>[4x]MGGSEIPMSEKTTKGVQLLRGDPKKAIVR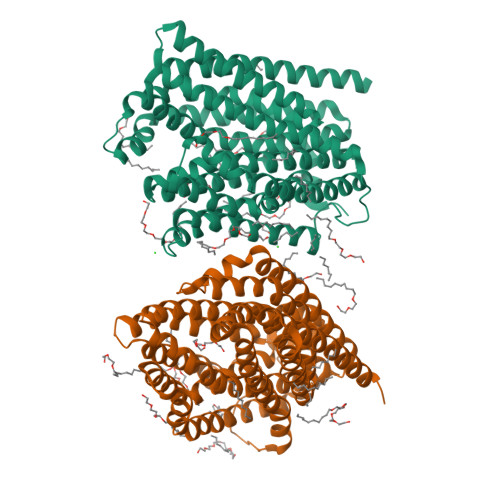LSIPMMIGMSVQTLYNLADGIWVSGLGPESLAAVGLFFPVFMGIIALAAGLGVGTSSAIARRIGARDKEGADNVAVHSLILSLILGVTITITMLPAIDSLFRSMGAKGEAVELAIEYARVLLAGAFIIVFNNVGNGILRGEGDANRAMLAMVLGSGLNIVLDPIFIYTLGFGVVGAAYATLLSMVVTSLFIAYWLFVKRDTYVDITLRDFSPSREILKDILRVGLPSSLSQLSMSIAMFFLNSVAITAGGENGVAVFTSAWRITMLGIVPILGMATATTSVTGAAYGERNVEKLETAYLYAIKIAFMIELAVVAFIMLFAPQVAYLFTYSESAQVIKGDLISALRTLPVFLVLTPFGMMTSAMFQGIGEGEKSLILTIFRTLVMQVGFAYIFVHYTTLGLRGVWIGIVIGNMVAAIVGFLWGRMRISALKKTSATGGKRRNSENLYFQGGRGSHHHHHHHHHH undeca-2-one coenzyme A | C32 H56 N7 O17 P3 S | 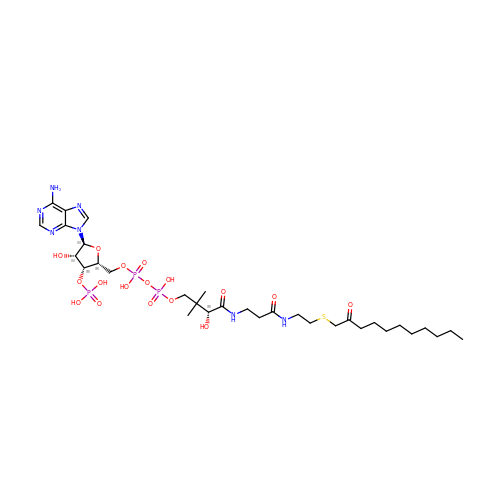JYQFMIDTWJSOBJ-BDQXTIGLSA-N>[3x]MDKSKLSVDPVIPNLYRKAREEGISTVFDRYEAQQPQCGFGLTGLCCRHCVQGPCRIDPFGEGPQAGICGATAEVITARNLLRQVTAGAAAHVDHAYDVLEVLEQIAQGTESYSIKDQEKLKQVAFTLGIDTANKTEQEIVEEMCQIIYRDFANSGATPMTYLKANSPRERLETWEKLGVLPRNPDREIREALHQTTMGMDADPVNLILKTIRLGLVDGFAGLKLATDLQDIIFGTPQPVVTEANLGVLKEDYVNIIVHGHVPLLSEKIVEWSRKLEDEAKKAGAKGINLAGICCTGNEVLMRQGVPLATNFLAQELAIITGAVDLMVVDVQCIMPSLAEIAACYHTRLVTTMPIVKIPGAEHVPFTTETADEASQQIVRMAIESYQKRNPAKVYIPREKAKVVAGFSVEAIVKALAKLNPDDPLKPLIDNIVSGNILGVVA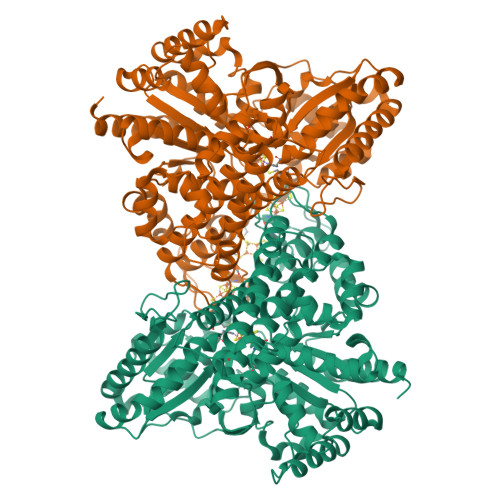TVGCNNVKVKHDWFHIELVKELIKNNVLVVTTGCSAHALAKAGLMDPAAAEWAGEGLRAVLTAIGTANDLGGPLPPVLHMGSCVDNSRIGDLVIAVANYLKVSPKDLPIAASAPEYQHEKALSIGTWAVAMGIMTHLGVVPPVVGSSKVTRILTQDAEALIGGKFYVETDPYKAAAGIIEHIKAKRALLNL> GVDPVEAFAQNVLSKADVIQATGDAICIFRELQCLTPRGRYDIRIYPTFLHLHGKTFDYKIPYTTVLRLFLLPHKDQRQMFFVISLDPPIKQG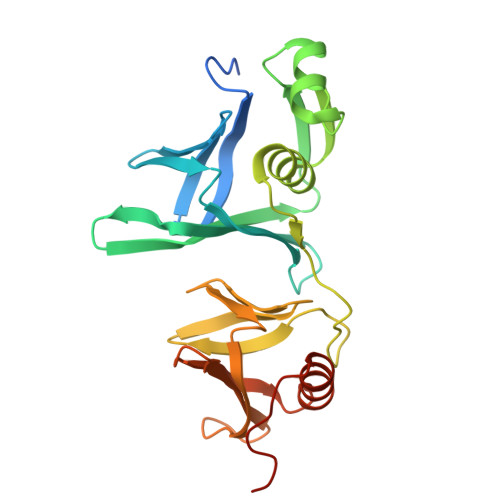QTRYHFLILLFSKDEDISLTLNMNEEEVEKRFEGRLTKNMSGSLYEMVSRVMKALVNRKITVPGNFQGHSGAQCITCSYKASSGLLYPLERGFIYVHKPPVHIRFDEISFVNFARGTTTTRSFDFEIETKQGTQYTFSSIEREEYGKLFDFVNAKKLNIKNRGLKEGMNPS Mutations in leucine-rich repeat kinase 2 (LRRK2) are one of the most common drivers of the familial form of Parkinson’s disease (PD) (1–3) and are also associated with increased risk for the sporadic form of PD. LRRK2 is a large, 2527-residue multidomain protein. Its N-terminal half is composed of armadillo (ARM), ankyrin (ANK), and leucine-rich (LRR) repeat domains, while its C-terminal half contains two catalytic domains, a guanosine triphosphatase (GTPase) (Ras of complex or ROC) and a Ser/Thr kinase, as well as two architectural domains, a C-terminal of ROC (COR) between the GTPase and the kinase and a WD40 domain at the end. We present cryo-EM structures of LRRK2RCKW, WT, and carrying the PD-linked mutations G2019S and I2020T, bound to the LRRK2-specific type I inhibitor MLi-2 or the broad-spectrum type II inhibitor GZD-824.

As with MLi-2, the three structures—WT, G2019S, and I2020T—were very similar. Although all three structures assumed a DYG “out”, αC “out” conformation with a broken R-spine and a disordered activation loop, the WT cryo-EM map showed a closer distance between K1906 and E1920. In all three cases, the G-loop was folded over the inhibitor to interact with its pyrazolopyridine and Y2018 from the DYG motif. Here, however, the cryo-EM map for LRRK2RCKW(G2019S):GZD-824 could accommodate two rotamers for H1998, while WT showed density for a single rotamer. H1998 is parallel to F1890 in the WT structure, where it adopts the “up” rotamer (H). A potential role for H1998 in the GZD-824–bound structures is in the stabilization of F1890 in the G-loop, which is packed against the pyrazolopyridine ring of the inhibitor. In this case, the cryo-EM map of LRRK2RCKW(G2019S):GZD-824 showed density indicative of two rotamers for H1998, only one of which would contribute to inhibitor binding, while we only saw the latter in the cryo-EM map of the WT complex. The prediction, based on this structural difference, that LRRK2(WT) might bind more tightly than G2019S to GZD-824 was consistent with in vitro measurements of the IC50 values for GZD-824 for these two variants.

> MASGSCQGCEEDEETLKKLIVRLNNVQEGKQIETLVQILEDLLVFTYSERASKLFQGKNIHVPLLIVLDSYMRVASVQQVGWSLLCKLIEVCPGTMQSLMGPQDVGNDWEVLGVHQLILKMLTVHNASVNLSVIGLKTLDLLLTSGKITLLILDEESDIFMLIFDAMHSFPANDEVQKLGCKALHVLFERVSEEQLTEFVENKDYMILLSALTNFKDEEEIVLHVLHCLHSLAIPCNNVEVLMSGNVRCYNIVVEAMKAFPMSERIQEVSCCLLHRLTLGNFFNILVLNEVHEFVVKAVQQYPENAALQISALSCLALLTETIFLNQDLEEKNENQENDDEGEEDKLFWLEACYKALTWHRKNKHVQEAACWALNNLLMYQNSLHEKIGDEDGHFPAHREVMLSMLMHSSSKEVFQASANALSTLLEQNVNFRKILLSKGIHLNVLELMQKHIHSPEVAESGCKMLNHLFEGSNTSLDIMAAVVPKILTVMKRHETSLPVQLEALRAILHFIVPGMPEESREDTEFHHKLNMVKKQCFKNDIHKLVLAALNRFIGNPGIQKCGLKVISSIVHFPDALEMLSLEGAMDSVLHTLQMYPDDQEIQCLGLSLIGYLITKKNVFIGTGHLLAKILVSSLYRFKDVAEIQTKGFQTILAILKLSASFSKLLVHHSFDLVIFHQMSSNIMEQKDQQFLNLCCKCFAKVAMDDYLKNVMLERACDQNNSIMVECLLLLGADANQAKEGSSLICQVCEKESSPKLVELLLNSGSREQDVRKALTISIGKGDSQIISLLLRRLALDVANNSICLGGFCIGKVEPSWLGPLFPDKTSNLRKQTNIASTLARMVIRYQMKSAVEEGTASGSDGNFSEDVLSKFDEWTFIPDSSMDSVFAQSDDLDSEGSEGSFLVKKKSNSISVGEFYRDAVLQRCSPNLQRHSNSLGPIFDHEDLLKRKRKILSSDDSLRSSKLQSHMRHSDSISSLASEREYITSLDLSANELRDIDALSQKCCISVHLEHLEKLELHQNALTSFPQQLCETLKSLTHLDLHSNKFTSFPSYLLKMSCIANLDVSRNDIGPSVVLDPTVKCPTLKQFNLSYNQLSFVPENLTDVVEKLEQLILEGNKISGICSPLRLKELKILNLSKNHISSLSENFLEACPKVESFSARMNFLAAMPFLPPSMTILKLSQNKFSCIPEAILNLPHLRSLDMSSNDIQYLPGPAHWKSLNLRELLFSHNQISILDLSEKAYLWSRVEKLHLSHNKLKEIPPEIGCLENLTSLDVSYNLELRSFPNEMGKLSKIWDLPLDELHLNFDFKHIGCKAKDIIRFLQQRLKKAVPYNRMKLMIVGNTGSGKTTLLQQLMKTKKSDLGMQSATVGIDVKDWPIQIRDKRKRDLVLNVWDFAGREEFYSTHPHFMTQRALYLAVYDLSKGQAEVDAMKPWLFNIKARASSSPVILVGTHLDVSDEKQRKACMSKITKELLNKRGFPAIRDYHFVNATEESDALAKLRKTIINESLNFKIRDQLVVGQLIPDCYVELEKIILSERKNVPIEFPVIDRKRLLQLVRENQLQLDENELPHAVHFLNESGVLLHFQDPALQLSDLYFVEPKWLCKIMAQILTVKVEGCPKHPKGIISRRDVEKFLSKKRKFPKNYMSQYFKLLEKFQIALPIGEEYLLVPSSLSDHRPVIELPHCENSEIIIRLYEMPYFPMGFWSRLINRLLEISPYMLSGRERALRPNRMYWRQGIYLNWSPEAYCLVGSEVLDNHPESFLKITVPSCRKGCILLGQVVDHIDSLMEEWFPGLLEIDICGEGETLLKKWALYSFNDGEEHQKILLDDLMKKAEEGDLLVNPDQPRLTIPISQIAPDLILADLPRNIMLNNDELEFEQAPEFLLGDGSFGSVYRAAYEGEEVAVKIFNKHTSLRLLRQELVVLCHLHHPSLISLLAAGIRPRMLVMELASKGSLDRLLQQDKASLTRTLQHRIALHVADGLRYLHSAMIIYRDLKPHNVLLFTLYPNAAIIAKIADYGIAQYCCRMGIKTSEGTPGFRAPEVARGNVIYNQQADVYSFGLLLYDILTTGGRIVEGLKFPNEFDELEIQGKLPDPVKEYGCAPWPMVEKLIKQCLKENPQERPTSAQVFDILNSAELVCLTRRILLPKNVIVECMVATHHNSRNASIWLGCGHTDRGQLSFLDLNTEGYTSEEVADSRILCLALVHLPVEKESWIVSGTQSGTLLVINTEDGKKRHTLEKMTDSVTCLYCNSFSKQSKQKNFLLVGTADGKLAIFEDKTVKLKGAAPLKILNIGNVSTPLMCLSESTNSTERNVMWGGCGTKIFSFSNDFTIQKLIETRTSQLFSYAAFSDSNIITVVVDTALYIAKQNSPVVEVWDKKTEKLCGLIDCVHFLREVMVKENKESKHKMSYSGRVKTLCLQKNTALWIGTGGGHILLLDLSTRRLIRVIYNFCNSVRVMMTAQLGSLKNVMLVLGYNRKNTEGTQKQKEIQSCLTVWDINLPHEVQNLEKHIEVRKELAEKMRRTSVE> ETRECKEALAKSEMNVNMKCQLPNFTAETPIQNVILHEHHIFLGATNYIYVLNEEDLQKVAEYKTGPVLEHPDCFPCQDCSSKANLSGGVWKDNINMALVVDTYYDDQLISCGSVNRGTCQRHVFPHNHTADIQSEVHCIFSPQIEEPSQCPDCVVSALGAKVLSSVKDRFINFFVGNTINSSYFPDHPLHSISVRRLKETKDGFMFLTDQSYIDVLPEFRDSYPIKYVHAFESNNFIYFLTVQRETLDAQTFHTRIIRFCSINSGLHSYMEMPLECILTEKRKKRSTKKEVFNILQAAYVSKPGAQLARQIGASLNDDILFAVFAQSKPDSAEPMDRSAMCAFPIKYVNDFFNKIVNKNNVRCLQHFYGPNHEHCFNRTLLRNSSGCEARRDEYRTEFTTALQRVDLFMGQFSEVLLTSISTFIKGDLTIANLGTSEGRFMQVVVSRSGPSTPHVNFLLDSHPVSPEVIVEHTLNQNGYTLVITGKKITKIPLNGLGCRHFQSCSQCLSAPPFVQCGWCHDKCVRSEECLSGTWTQQICLPAIYKVFPNSAPLEGGTRLTICGWDFGFRRNNKFDLKKTRVLLGNESCTLTLSESTMNTLKCTVGPAMNKHFNMSIIISNGHGTTQYSTFSYVDPVITSISPKYGPMAGGTL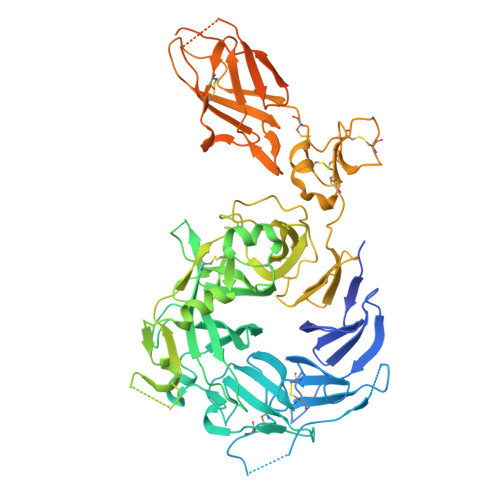LTLTGNYLNSGNSRHISIGGKTCTLKSVSNSILECYTPAQTISTEFAVKLKIDLANRETSIFSYREDLHHHHHH>GPGFDFAQAIMKKNTVIARTEKGEFTMLGVYDRVAVIPTHASVGETIYINDVETKVLDACALRDLTDTNLEITIVKLDRNQKFRDIRHFLPRYEDDYNDAVLSVHTSKFPNMYIPVGQVTNYGFLNLGGTPTHRILMYNFPTRAGQAGGVVTTTGKVIGIHVGGNGAQGFAAMLLHSYFSDTQ[2x]

During viral replication of EV68, the viral genome is translated into a single, large polyprotein comprised of structural and non-structural proteins. The viral polyprotein needs to be cleaved into individual proteins for viral replication to proceed. The 3C protease cleaves eight sites in the polyprotein with a preference for a glutamine–glycine (QG) motif at the P1/P1′ positions. The conserved essential function in viral replication makes the 3C protease a promising target for DAA development.

We also determined a high-resolution apo structure of the inactive C147A mutant EV68-3C protease for comparison. The C-alpha distances between the two structures were calculated and the average for each residue mapped onto the two structures (ranging from 0 Å to 1.5 Å). The largest variation was observed around the active site, at the P1 binding pocket. In the apo structure, the areas surrounding the P1 glutamine binding pocket form a narrow and more open channel. With the apo and peptide-bound co-crystal structures with a viral cleavage site of the EV68-3C, we were also able to characterize the large conformational changes that occur upon substrate binding.>GPHMDKAYFIAKEVSTTERTYLKDLEVITSWFQSTVSKEDAMPEALKSLIFPNFEPLHKFHTNFLKEIEQRLALWEGRSNAQIRDYQRIGDVMLKNIQGMKHLAAHLWKHSEALEALENGIKSSRRLENFCRDFELQKVCYLPLNTFLLRPLHRLMHYKQVLERLCKHHPPSHADFRDCRAALAEITEMVAQLHGTMIKMENFQKLHELKKDLIGIDNLVVPGREFIRLGSLSKLSGKGLQQRMFFLFNDVLLYTSRGLTASNQFKVHGQLPLYGMTIEESEDEWGVPHCLTLRGQRQSIIVAASSRSEMEKWVEDIQMAIDLAEKSSSPAP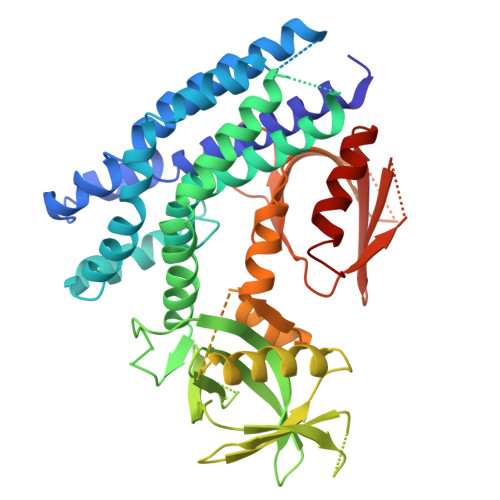EFLASSPPDNKSPDEATAADQESEDDLSASRTSLERQAPHRGNTMVHVCWHRNTSVSMVDFSIAVENQLSGNLLRKFKNSNGWQKLWVVFTNFCLFFYKSHQDNHPLASLPLLGYSLTIPSESENIQKDYVFKLHFKSHVYYFRAESEYTFERWMEVIRSATSSASRPH[2x]> MTGDHIKVIYFNGRGRAESIRMTLVAAGVNY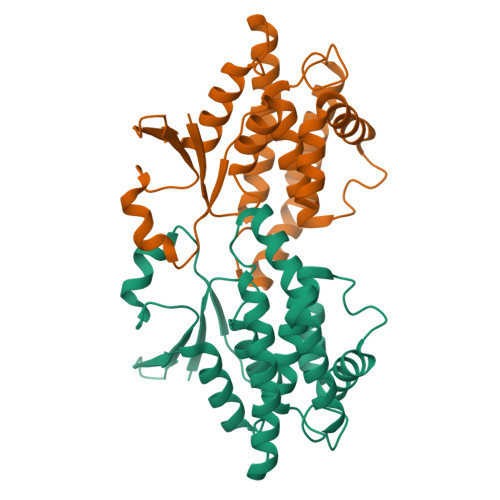EDERISFQDWPKIKPTIPGGRLPAVKITDNHGHVKWMLESLAIARYMAKKHHMMGETDEEYYNVEKLIGQVEDLEHEYHKTLMKPEEEKQKITKEILNGKVPVLLDIICESLKASTGKLAVGDKVTLADLVLIAVIDHVTDLDKEFLTGKYPEIHKHRENLLASSPRLAKYLSDRAATPF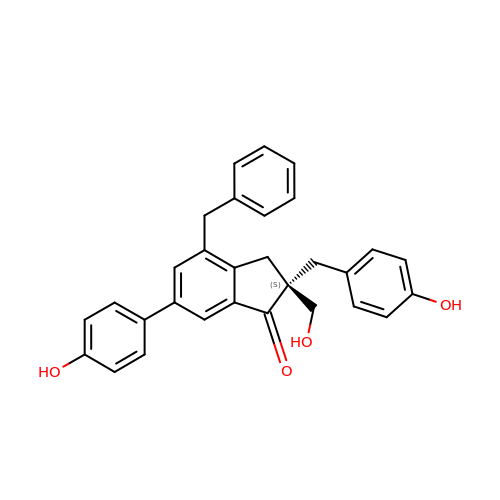(2~{S})-2-(hydroxymethyl)-6-(4-hydroxyphenyl)-2-[(4-hydroxyphenyl)methyl]-4-(phenylmethyl)-3~{H}-inden-1-one | C30 H26 O4 | OCWYWPXFECTDDD-PMERELPUSA-N>MQKVEVFRIPTASPDDISG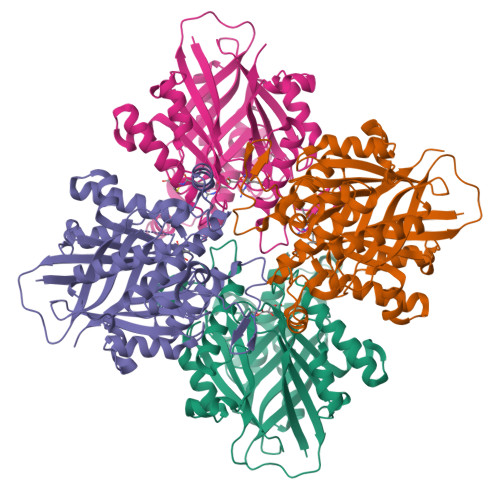LATLIDSGKINPAEIVAILGKTEGNGSVNDFTRCFATQSLAMYLAEKLGISREEVVKKVAFIMSGGTEGVMTPHITVFVRKDVAAPAAPGKRLAVGVAFTRDFLPEELGRMEQVNEVARAVKEAMKDAQIDDPRDVHFVQIKAPLLTAERIEDAKRRGKDVVVNDTYKSMAYSRGASALGVALALGEISADKISNEAIVHDWNLYSSVASTSAGVCLLNDEIIVVGNSTNSASDLVIGHSVMKDAIDADAVRAALKDAGIRSDDEMDRIVNVLAKAEAASSGTVRGRRNTMLDDSDINHTRSARAVVNAVIASVVGDPMVYVSGGAEHQGPDGGGPIAVIARVLEHHHHHH[8x]>GFLSGKRILVT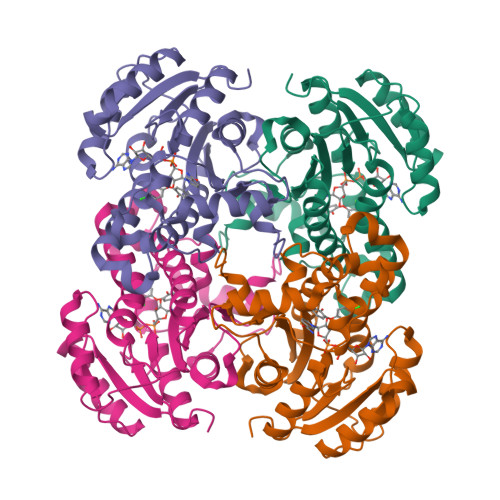GVASKLSIAYGIAQAMHREGAELAFTYQNDKLKGRVEEFAAQLGSDIVLQCDVAEDASIDTMFAELGKVWPKFDGFVHSIGFAPGDQLDGDYVNAVTREGFKIAHDISSYSFVAMAKACRSMLNPGSALLTLSYLGAERAIPNYNVMGLAKASLEANVRYMANAMGPEGVRVNAISAGPIRTLAASGIKDFRKMLAHCEAVTPIRRTVTIEDVGNSAAFLCSDLSAGISGEVVHVDGGFSIAAMNELELK[4x]> GSMFGCLVAGRLVQTAAQQVAEDK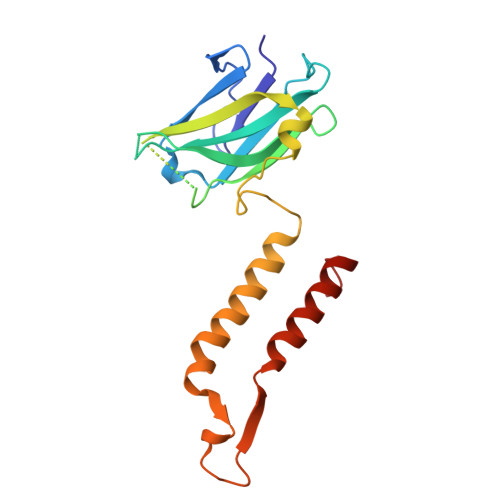FVFDLPDYESINHVVVFMLGTIPFPEGMGGSVYFSYPDSNGMPVWQLLGFVTNGKPSAIFKISGLKSGEGSQHPAGAMNIVRTPSVAQIGISVELLDSMAQQTPVGNAAVSSVDSFTQFTQKMLDNFYNFASSFAVSQAQMTPSPSEMFIPANVVLKWYENFQRRLAQNPLFWKT> MKESLMD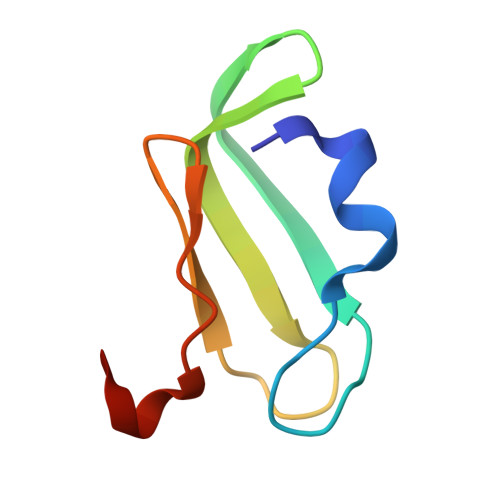ILCDPLDKSELELEVDERDGDEIIEGRLIGTVTGEVYPIEDGIPNLLPPDMRDD> MKSKNGVPFGLLSGIFWGLGLTVSAYIFSIFTDLSPFVVAATHDFLSIFILLAFLLVKEGKVRLSIFLNIRNVSVIIGALLAGPIGMQANLYAVKYIGSSLASSVSAIYPAISVLLAFFFLKHKISKNTV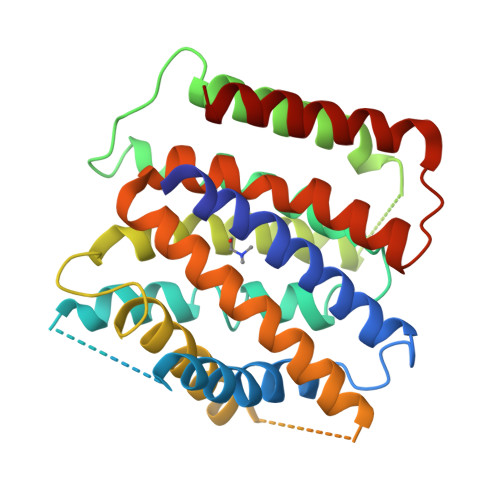FGIVLIIGGIIAQTYKVEQVNSFYIGILCALVCAIAWGSESVLSSFAMESELSEIEALLIRQVTSFLSYLVIVLFSHQSFTAVANGQLLGLMIVFAAFDMISYLAYYIAINRLQPAKATGLNVSYVVWTVLFAVVFLGAPLDMLTIMTSLVVIAGVYIIIKE>[4x]EETPVTPQPPDILLGPLFNDVQNAKLFPDQKTFADAVPNSDPLMILADYRM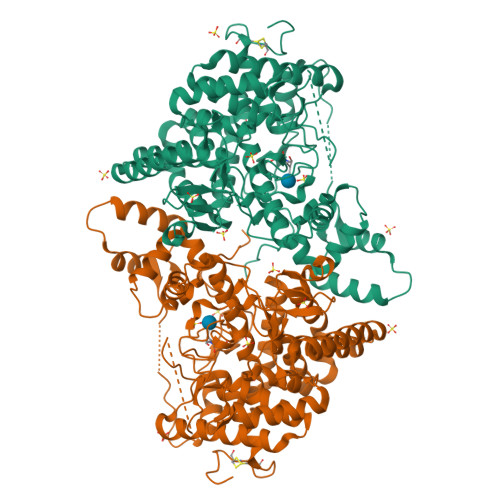QQNQSGFDLRHFVNVNFTLPKEGEKYVPPEGQSLREHIDGLWPVLTRSTENTEKWDSLLPLPEPYVVPGGRFREVYYWDSYFTMLGLAESGHWDKVADMVANFAHEIDTYGHIPNGNRSYYLSRSQPPFFALMVELLAQHEGDAALKQYLPQMQKEYAYWMDGVENLQAGQQEKRVVKLQDGTLLNRYWDDRDTPRPESWVEDIATAKSNPNRPATEIYRDLRSAAASGWDFSSRWMDNPQQLNTLRTTSIVPVDLNSLMFKMEKILARASKAAGDNAMANQYETLANARQKGIEKYLWNDQQGWYADYDLKSHKVRNQLTAAALFPLYVNAAAKDRANKMATATKTHLLQPGGLNTTSVKSGQQWDAPNGWAPLQWVATEGLQNYGQKEVAMDISWHFLTNVQHTYDREKKLVEKYDVSTTGTGGGGGEYPLQDGFGWTNGVTLKMLDLICPKEQPCDNVPATRPTVKSATTQPSTKEAQPTP alpha-zearalanol | C18 H26 O5 | 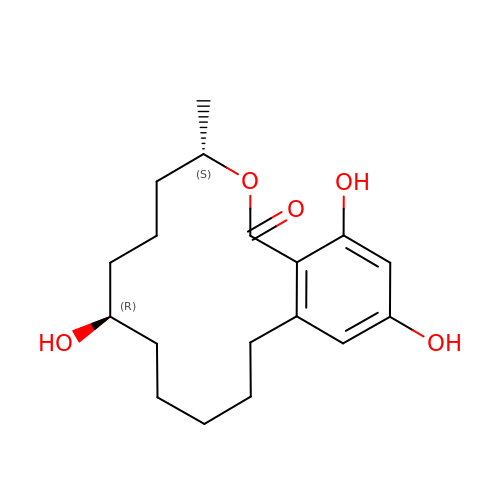DWTTZBARDOXEAM-GXTWGEPZSA-N>GAMGSGMAMDTFITRNFQTTIIQKAKNTMAEFSEDPELQPAMLFNICVHLEVCYVISDMNFLDEEGKSYTALEGQGKEQNLRPQYEVIEGMPRTIAWMVQRSLAQEHGIETPKYLADLFDYKTKRFIEVGITKGLADDYFWKKKE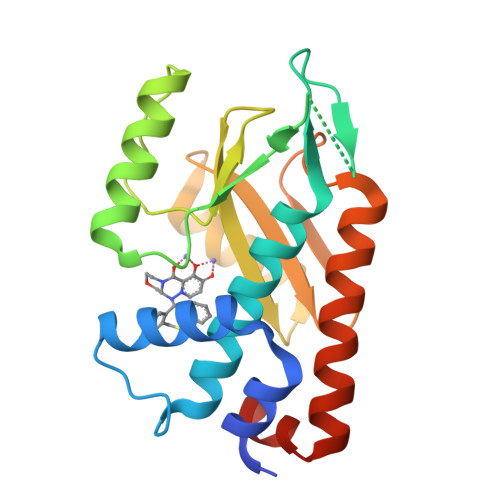KLGNSMELMIFSYNQDYSLSNESSLDEEGKGRVLSRLTELQAELSLKNLWQVLIGEEDVE[2x]>SDAPNFVLEDTNGKRIELSDLKGKGVFLNFWGTWCEHCKKEFPYMANQYKHFKSQGVEIVAVNVGESKIAVHNFMKSYGV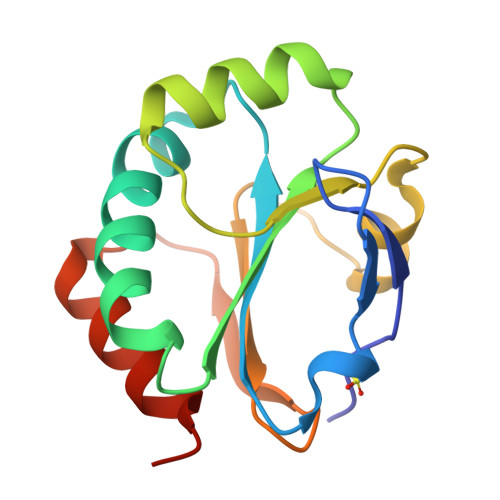NFPVVLDTDRQVLDAYDVSPLPTTFLINPEGKVVKVVTGTMTESMIHDYMNLIKPGETSG[2x]The genome of S. pneumoniae contains genes that encode a suite of proteins that are biochemically capable of performing the various concerted steps needed to completely depolymerize and transport all classes of N-glycans found on host glycoconjugates. Here we characterize SpGH92 (TIGR4 locus tag SP_2145) as an α-mannosidase that trims the terminal α-(1,2)-linked mannose residues on high-mannose glycans to generate a substrate for EndoD. We also identify a solute binding protein (SBP; NgtS) from an ABC transporter (ABCNG) that binds soluble N-glycans and, through X-ray crystallography, reveal the molecular basis of its interaction with these branched glycans. The identification of an ABC transporter that possesses an SBP, NgtS, that is specific to the recognition of N-glycan fragments suggests that this is likely the convergence point of the complex and high mannose N-glycan processing sides of the N-glycan degradation pathway, with this transporter functioning to import soluble N-glycan fragments into the bacterium.

ITC using Man5GlcNAc as a ligand gave an association constant (Ka) of 1.04 (± 0.01)×106 M−1, which is consistent with the range of affinities previously determined for other SBPs, and a binding stoichiometry of 1.05 (±0.01), equating to the expected 1:1 protein to ligand ratio. Despite these two complexes being obtained with different ligands and in different spacegroups, the overall conformations of NgtS were very similar (rmsd of 1.0 Å over 427 matched Cα positions); both complexes were in a “closed” conformation relative to the “open” conformation obtained in the absence of ligand. As with other SBPs, the ligand-binding site was found at the interface of the two domains comprising NgtS and ligand recognition involves a transition from the open, unbound form to a ligand-stabilized closed form. The reducing end of the carbohydrate is oriented into the base of the protein binding cleft and fully sequestered from bulk solvent with no room for additional residues present at the reducing end, consistent with our proposal that NgtS specifically binds the products of EndoD hydrolysis (i.e. having only the single non-reducing GlcNAc residue). The additional α-(1,3)- and α-(1,6)-linked mannose residues of Man5GlcNAc provide a number of direct hydrogen bond interactions with the protein and an extensive network of water mediated hydrogen bonds. The classic CH-π interaction between aromatic sidechains and carbohydrate rings, such as that seen in binding the Man1GlcNAc core, is notably absent between the protein and the mannose residues in the glycan arms, though Trp81 does participate in hydrogen bonding with the terminal α-1,6-linked mannose. The structure of NgtS in complex with this ligand revealed a specific network of interactions, with the suite of interactions between the reducing end GlcNAc residue and the burial of this sugar at the base of the binding site imparting specificity for the reducing end motif glycans.

>[4x]MGNLTGNSKKAADSGDKPVIKMYQIGDKPDNLDELLANANKIIEEKVGAKLDIQYLGWGDYGKKMSVITSSGENYDIAFADNYIVNAQKGAYADLTELYKKEGKDLYKALDPAYIKGNTVNGKIYAVPVAANVASSQNFAFNGTLLAKYGIDISGVTSYETLEPVLKQIKEKAPDVVPFAIGKVFIPSDNFDYPVANGLPFVIDLEGDTTKVVNRYEVPRFKEHLKTLHKFYEAGYIPKDVATSDTSFDLQQDTWFVREETVGPADYGNSLLSRVANKDIQIKPITNFIKKNQTTQVANFVISNNSKNKEKSMEILNLLNTNPELLNGLVYGPEGKNWEKIEGKENRVRVLDGYKGNTHMGGWNTGNNWILYINENVTDQQIENSKKELAEAKESPALGFIFNTDNVKSEISAIANTMQQFDTAINTGTVDPDKAIPELMEKLKSEGAYEKVLNEMQKQYDEFLKNKKLEHHHHHH>[24x]GASGSGTGSGSMSTLYLTQPDAVLSKKHEAFHVALKQEDGSWKKQPIPAQTLEDIVLLGYPSITGEALGYALELGLPVHYLTQFGKYVGSALPSESRNGQLRLAQFRAHEDPIQRLDIVKAFVKGKVHNQYNLLYRRGQVDNPLKGRGKLVMRQQTLEQVRGIEGLAAREYFASWQEMLGHEWTFTGRFRRPPTDPVNALLSFGYGLLRTQ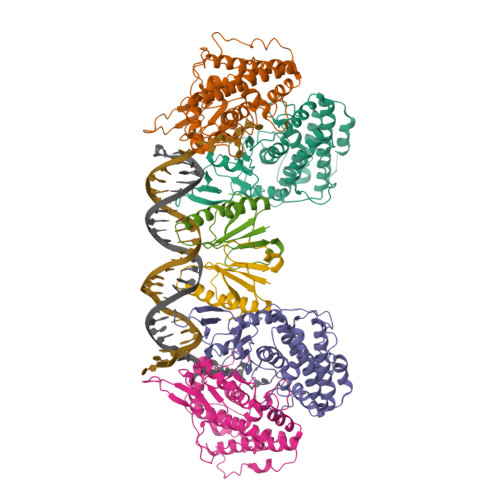VTAAVHIAGLDPYIGFLHETTRGQPAMILDLMEEFRALVADSVVLTVLKQREIQRQDFTESLGAFRLTDSATKTFLGAFDRKLSSEFKHPIFNYKCTYRRAIELQARLLARHLQEGVVYEPLVIR;>[12x]GASGSGTGSGSMLYLIIYDVPATKAGNKRRTRLFDLLSGYGKWRQFSVFECFLSVKQFAKLQTAMEKLIKLDEDAVCIYVLDENTVQRTITYGTPQPEKPGSIII> MEYTFNKLTKKDVKKLKVGDIVYLNGKIYTARDEAHLKIIEMLKSNEKLPFDLNESIIYHAGPIMKKVNDSWVCVSIGPTTSARMNDVEEEFIKLTNISAIVGKGGMKKELLKTFEDYGVVYLAAPGGCAALLANSVKRVDNVYFLDELGMPEAVWELEVNNFGPLIV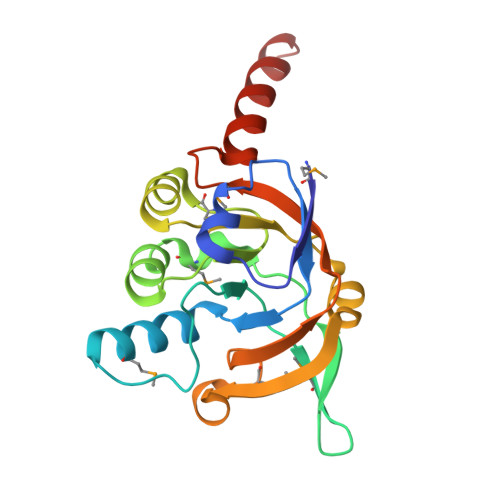AMDSHGNSIYEEVNKKVYEKLNELIGL We have biochemically and structurally characterized a minimalist inositol phosphate kinase (i.e., TvIPK) encoded by Terrestrivirus, a nucleocytoplasmic large (“giant”) DNA virus (NCLDV). We show that TvIPK can synthesize inositol pyrophosphates from a range of scyllo- and myo-IPs, both in vitro and when expressed in yeast cells. We find a heart-shaped ligand binding pocket comprising an array of positively charged and flexible side chains, underlying the observed substrate diversity. A crucial arginine residue in a conserved “G-loop” orients the γ-phosphate of ATP to allow substrate pyrophosphorylation.

For each asymmetric unit, there is one molecule of TvIPK17-265 in the C2221 space group. The N-terminal residues 17–47 could not be traced, either in this crystal complex, or in a binary complex of full-length TvIPK plus ADP, or in a number of TvIPK17-265/ADP complexes into which we soaked a variety of inositol phosphates (Table EV1, B and EV2A).

> MSITDMPNMANIANMADITNMSNIDLQSSKSVADEVIADIAEIVNKESIRIFPRIAGRSYIIYGQTSGIICKRMEKSDNEFVIYNYISEHYDKFLKKYVPKLYGKNNDMLLLEDLTYNYNNPNVMDVKIGARKRKSHTSGFFSIRGYTNSHDYKFDPDEYLTSESTINHIKNFMEAGGENRDKTKQVLLKWIMKLSELANDLFEINLKFDGVSLIFIYDDDCSKCDVNVVDFSRVKLIDTNDQMTISAVTNLIKILSELADNPLN> MHHHHHHDDDDKAMGANTEAQGSGRGLEAMKWVVVVALLLVAIVGNYLYRDIMLPLRALAVVILIAAAGGVALLTTKGKATVAFAREARTEVRKVIWPT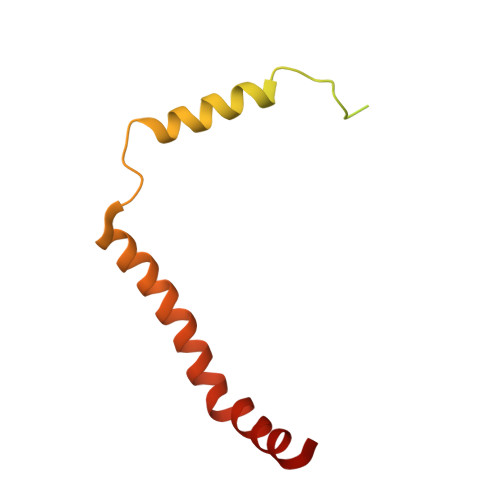RQETLHTTLIVAAVTAVMSLILWGLDGILVRLVSFITGLRF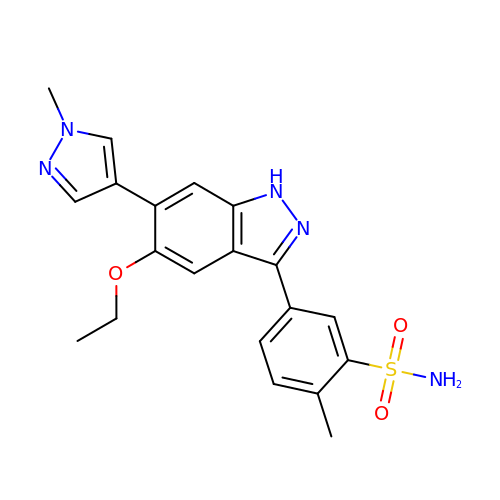5-[5-ethoxy-6-(1-methyl-1H-pyrazol-4-yl)-1H-indazol-3-yl]-2-methylbenzenesulfonamide | C20 H21 N5 O3 S | CITPEYUXGCJVRV-UHFFFAOYSA-N N-[TOSYL-D-PROLINYL]AMINO-ETHANETHIOL | C14 H20 N2 O3 S2 | 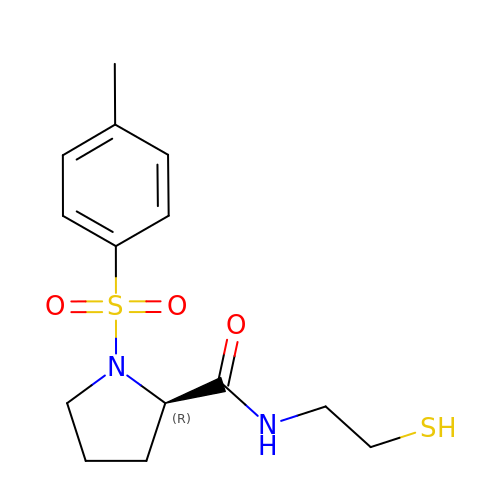NWUYDTGYTUQMDG-CYBMUJFWSA-N DEP domain-containing mTOR interacting protein (DEPTOR), conserved in vertebrates, modulates the activity of the serine/threonine kinase mammalian target of rapamycin (mTOR), a master regulator of cell growth. mTOR acts in two functionally distinct multiprotein complexes, mTOR complex 1 (mTORC1) and mTORC2, and DEPTOR is the only protein reported to bind and inhibit both mTOR complexes. DEPTOR is a 46 kDa protein comprising an N-terminal DEP (Dishevelled, Egl-10, and Pleckstrin) domain tandem, herein referred to as DEPt, and a C-terminal PDZ (postsynaptic density 95, disks large, zonula occludens-1) domain. Biochemical analysis and cryo-EM reconstructions of DEPTOR bound to human mTOR complex 1 (mTORC1) and mTORC2 reveal that both structured regions of DEPTOR, the PDZ domain and the DEP domain tandem (DEPt), are involved in mTOR interaction. The PDZ domain binds tightly with mildly activating effect, but then acts as an anchor for DEPt association that allosterically suppresses mTOR activation.

To obtain a pseudo-atomic model of the second DEPTOR-mTOR binding interface, we determined an X-ray crystal structure of a recombinant DEPt region (aaDEPTOR 1–230) at 1.93 Å resolution in a domain-swapped conformation as revealed by small-angle X-ray scattering (SAXS) in solution. Each of the two domains in DEPt adopts a characteristic DEP domain fold comprising an alpha-helical core and a protruding beta-hairpin arm. In the DEPt, the two DEP domains are interacting via their N-terminal alpha-helices and a C-terminal extension of the second DEP domain that folds back onto the first DEP domain. (b) The DEPt of DEP domain-containing mTOR interacting protein (DEPTOR) crystallized as a domain-swapped dimer. The domain-swapped dimer is stabilized by a non-native disulfide bridge between C102 of the protomers. The DEPt is monomeric in solution in a conformation corresponding to the conformation found in the crystal structure, which is related to the mTOR-bound state by a simple domain rotation with minor translation component. Binding of DEPt to mTOR preserves the overall fold of DEPt, but is linked to a 3.6 Å translation and 39° rotation between the two DEP domains. DEP1 of DEPt, which mainly mediates interaction of DEPt and mTOR, is more conserved than DEP2. The two positively charged patches in DEPt were recently described to bind to phosphatidic acid (PA).

>[2x]MEEGGSTGSAGSDSSTSGSGGAQQRELERMAEVLVTGEQLRLRLHEEKVIKDRRHHLKTYPNCFVAKELIDWLIEHKEASDRETAIKLMQKLADRGIIHHVCDEHKEFKDVKLFYRFRKDDGTFPLDNEVKAFMRGQRLYEKLMSPENTLLQPREEEGVKYERTFMASEFLDWLVQEGEATTRKEAEQLCHRLMEHGIIQHVSSKHPFVDSNLLYQFRMNFRRRRRLMEL>[4x]MKIAVIGQSLFGQEVYCQLRKEGHEVVGVFTIPDKDGKADPLGLEAEKDGVPVFKFPRWRARGQALPEVVAKYQALGAELNVLPFCSQFIPMEVINAPRHGSIIYHPSLLPRHRGASAINWTLIHGDKKGGFTIFWADDGLDTGDLLLQKECEVLPDDTVSTLYNRFLFPEGIKGMVQAVRLIAEGTAPRCPQSEEGATYEGIQKKETAKINWDQPAEAIHNWIRGNDKVPG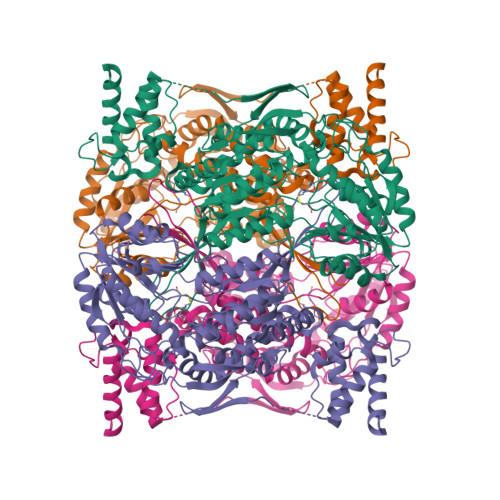AWTEACGQKLTFFNSTLNTSGLSTQGEALPIPGAHRPGVVTKAGLILFGNDDRMLLVKNIQLEDGKMMPASQFFKGSASSDLELTEAELATAEAVRSSWMRILPNVPEVEDSTDFFKSGAASVDVVRLVEEVKELCDGLELENEDVYMATTFRGFIQLLVRKLRGEDDESECVINYVEKAVNKLTLQMPYQLFIGGEFVDAEGSKTYNTINPTDGSVICQVSLAQVSDVDKAVAAAKEAFENGLWGKINARDRGRLLYRLADVMEQHQEELATIEALDAGAVYTLALKTHVGMSIQTFRYFAGWCDKIQGATIPINQARPNRNLTLTKKEPVGVCGIVIPWNYPLMMLSWKTAACLAAGNTVVIKPAQVTPLTALKFAELTLKAGIPKGVVNILPGSGSLVGQRLSDHPDVRKIGFTGSTEVGKHIMKSCALSNVKKVSLELGGKSPLIIFADCDLNKAVQMGMSSVFFNKGENCIAAGRLFVEESIHNQFVQKVVEEVEKMKIGNPLERDTNHGPQNHEAHLRKLVEYCQRGVKEGATLVCGGNQVPRPGFFFQPTVFTDVEDHMYIAKEESFGPIMIISRFADGDVDAVLSRANATEFGLASGVFTRDINKALYVSDKLQAGTVFINTYNKTDVAAPFGGFKQSGFGKDLGEAALNEYLRIKTVTFEY> GSHMPEPTVEDVISQVARAHREIFTYAHDKLGSSPGNFNANHASGSPHGRSGRTVQEIWEDFSMSFTPAVREVVEFAKHIPGFRDLSQHDQVTLLKAGTFEVLMVRFASLFNVKDQTVMFLSRTTYSLQELGAMGMGDLLSAMFDFSEKLNSLALTEEELGLFTAVVLVSADRSGMENSASVEQLQETLLRALRALVLKNRPLETSRFTKLLLKLPDLRT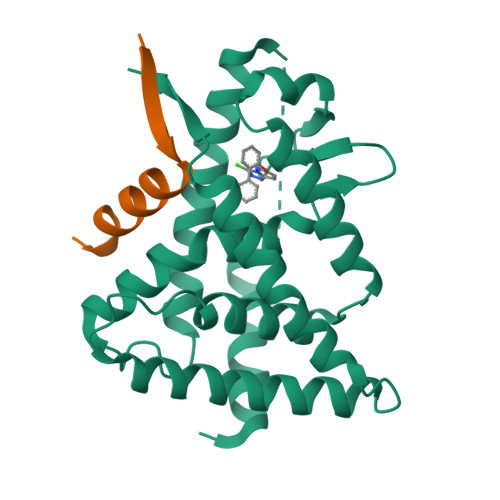LNNMHSEKLLSFRVDAQ;> THRLITLADHIAQIITQDFA An ABC transporter is a critical component of the Mla pathway, which is a phospholipid transport system that is important for outer membrane (OM) integrity in many Gram-negative species, and has been implicated in the Maintenance of outer membrane Lipid Asymmetry. Two copies of MlaF, an ABC ATPase, and two copies of MlaE, a multipass transmembrane protein, form an MlaF2E2 subcomplex that represents the conserved ABC transporter core. MlaB is stably associated with the cytoplasmic part of the transporter complex: one MlaB subunit binds to the side of each of the two MlaF ATPase domains. We and others have hypothesized that MlaB may regulate the MlaFEDB transporter complex, perhaps through its interaction with the MlaF ATPase. Here we report structures of the MlaFB complex, and present a model for how these two proteins may work together.

In contrast, the MlaF1B1 structure represents an inactive ‘half-transporter’, but will be discussed where it provides additional insights into unique features of the MlaF-MlaB interaction. Moreover, in the MlaF1B1 structure, which crystallized in a different space group (P212121) from that of MlaF2B2 (P3221) with completely different crystal packing, the MlaF CTE is ordered and the terminal helix is bound to neighboring MlaFB monomers in a similar conformation. Indeed, when our MlaF1B1 and MlaF2B2 structures are superimposed on the catalytic subdomain, we observe a rotation of the helical subdomain by ~10 degrees. Perhaps as a consequence of this subdomain rotation, the Q-loop is displaced from its usual location near the site of catalysis, consistent with its role in linking the site of ATP hydrolysis in the catalytic subdomain to the helical subdomain.

>[4x]MEQSVANLVDMRDVSFTRGNRCIFDNISLTVPRGKITAIMGPSGIGKTTLLRLIGGQIAPDHGEILFDGENIPAMSRSRLYTVRKRMSMLFQSGALFTDMNVFDNVAYPLREHTQLPAPLLHSTVMMKLEAVGLRGAAKLMPSELSGGMARRAALARAIALEPDLIMFDEPFVGQDPITMGVLVKLISELNSALGVTCVVVSHDVPEVLSIADHAWILADKKIVAHGSAQALQANPDPRVRQFLDGIADGPVPFRYPAGDYHADLLPGS;>MHHHHHHENLYFQSESLSWMQTGDTLALSGELDQDVLLPLWEMREEAVKGITCIDLSRVSRVDTGGLALLLHLIDLAKKQGNNVTLQGVNDKVYTLAKLYNLPADVLPR[4x]>FDDLRPRLGRLTEETIDIAREVLVEGKSQSDVARERGLSRQRVSSMVKSVVSAANEIPREWQRVEVWLPPNLAEKVRQMEADAKADVARKNQLTDAAL[2x]

ArdK is a 102 amino acid protein encoded by the broad host range conjugative plasmid R388. In R388, ArdK represses the expression of five genes by its binding to their respective promoters (PardC, Porf7, Pssb, Porf12 and Porf14). The KorA family of transcriptional regulators includes plasmid-borne repressors involved in plasmid stability and conjugation. Our structural analyses show that ArdK, a member of this family, can form a symmetric dimer similar to that observed for KorA, yet it binds direct sequence repeats as a non-symmetric dimer.

To study the binding mechanism of ArdK, we obtained the crystal structure of the protein bound to its cognate DNA operator. We chose the operator present in the Pssb promoter (GTATTGACACCTATTGACA; underlining indicates the –35 box), as this was the promoter with the highest level of repression by ArdK. Two complementary 19mer oligonucleotides containing this sequence were annealed and bound to SeMet ArdK, as described in the Materials and Methods. Crystals of the ArdK–DNA complex were obtained, and the structure solved at 2.8 Å resolution. In the ArdKSE–DR crystal structure, we found an ArdK dimer bound to a single dsDNA molecule within the asymmetric unit. Each of the DR repeats is bound by each of the ArdK HTH domains. The main residues involved in specific interactions with the recognized sequence were R45 and Q46. R45 NH2 interacted with G2_C or G12_C O6, R45 Nϵ with G2_C or G12_C N7, and Q46 Nϵ2 with G6_D or G16_D O6. Hydrogen bonds with the DNA backbone phosphates, and van der Waals forces stabilize the DNA interaction. To achieve this rather unusual binding architecture, one of the HTHs had to rotate 180° relative to its apo position, while the other HTH motif and the dimerization domain remained at their original position.>GDNPCAAGPPVDTNPAECCPKPMLVDGTIMMDCYKKYGEQTKKQLQMDGIPRGCCIAECAMNATNMYADGMLKRDDLSKMFMDAVKDKPEWMSLVRDATNACFELAEKKMDEIEAGAKLEPSFEGEKICHPISGTILRCMGMMMFAQ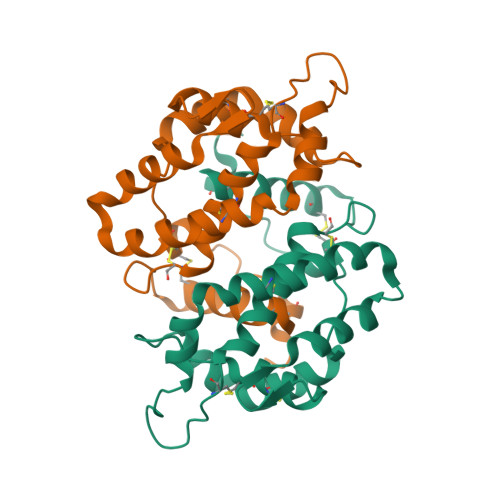CPASVFNVNENCNKLREYGSICPMI[4x]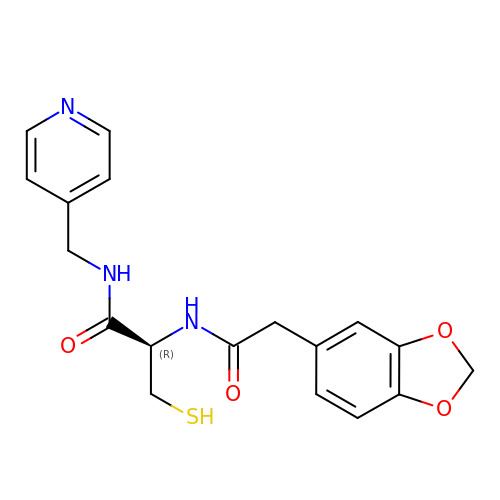N~2~-[(2H-1,3-benzodioxol-5-yl)acetyl]-N-[(pyridin-4-yl)methyl]-L-cysteinamide | C18 H19 N3 O4 S | PDIUERQHFJXFMT-AWEZNQCLSA-N N~2~-(4-cyano-3-methyl-1,2-thiazol-5-yl)-N~2~-methylglycinamide 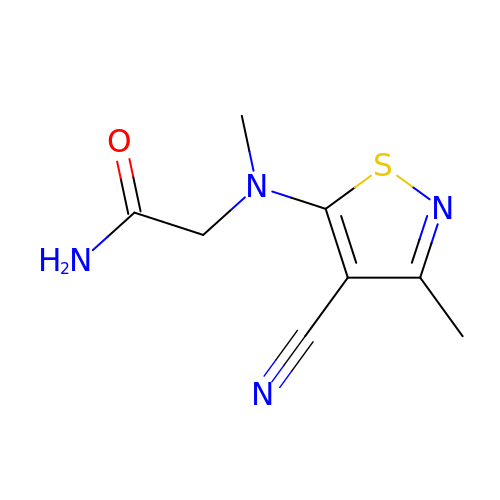| C8 H10 N4 O S | BCFQGXBWVPWHCV-UHFFFAOYSA-N> DPNEAVREFAKEIDVSYVKIEEVIGAGEFGEVCRGRLKAPGKKESCVAIKTLKGGYTERQRREFLSEASIMGQFEHPNIIRLEGVVTNSMPVMILTEFMENGALDSFLRLNDGQFTVIQLVGMLRGIASGMRYLAEMSYVHRDLAARNILVNSNLVCKVSDFGLSRFLEENSSDPTETSSLGGKIPIRWTAPEAIAFRKFTSASDAWSYGIVMWEVMSFGERPYWDMSNQDVINAIEQDYRLPPPPDCPTSLHQLMLDCWQKDRNARPRFPQVVSALDKMIR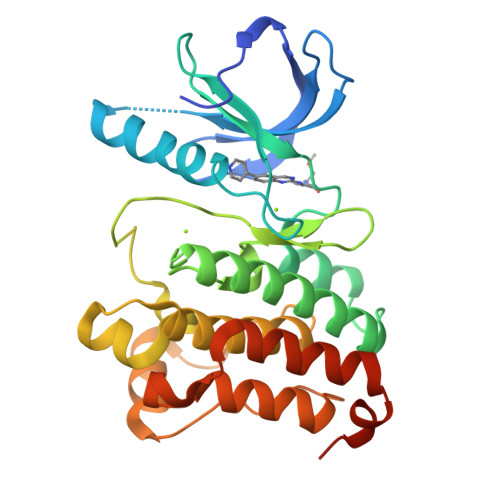NPASLKIVARENGGASHPLL>[3x]MQDYTVHIVDDEEPVRKSLAFM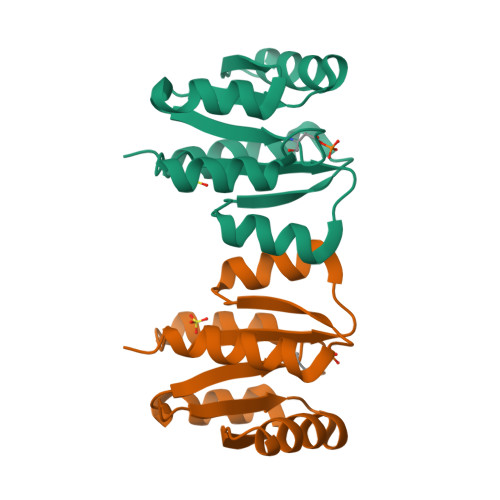LTMNGFAVKMHQSAEAFLAFAPDVRNGVLVTDLRMPDMSGVELLRNLGDLKINIPSIVITGHGDVPMAVEAMKAGAVDFIEKPFEDTVIIEAIERASEHLVALE The ESCRT-III-like protein Vipp1 couples filament polymerization with membrane remodeling. It assembles planar sheets as well as 3D rings and helical polymers, all implicated in mitigating plastid-associated membrane stress. PspA activity is triggered by agents that threaten inner membrane integrity, including phage, mislocalized secretins, and antibiotics, whereas Vipp1 is a plastid component in cyanobacteria, algae, and plants, in which it functions in thylakoid membrane biogenesis and repair. Given that two-dimensional (2D) planar sheets share a close geometric relationship with helical lattices, and as a means of understanding the interconnectedness of Vipp1 polymers including rings, spirals and planar sheets, we determined the structure of four Vipp1 helical filaments by cryo-EM.

Alternatively, Vipp1Δα61–219 assembled with related but different lattices, termed Vipp1Δα6_L2 and Vipp1Δα6_L3. Vipp1Δα6_L3 was the only lattice in which class averages of aligned particles yielded a Fourier Transform with non-overlapping layer lines amenable to indexing. Only helical parameters with a rise of 2.16 Å and a rotation of 85.50° yielded a 3.7 Å-resolution map, with excellent side chain detail enabling model building from amino acids 1–217. Map quality was lowest around the C terminus of helix 5 (α5C), indicative of instability within interface 1—a trait observed for all Vipp1 helical filaments, to differing degrees. Vipp1Δα6_L3 was 24.4 nm in diameter, with a hollow inner lumen that was 12.7 nm across. Specifically, Vipp1 formed ESCRT-III-like protofilaments, in which hairpin motifs packed side by side and the α5C of subunit j bound across the hairpin tip of subunit j+3 to form the classical interface 1 domain swop. These protofilaments formed a 17-start right-handed helix that ran diagonally around the helical axis. Concurrently, each hairpin tip bound the N terminus of helix 5 (α5N) in a neighboring protofilament, thereby forming interface 3. Neighboring protofilaments aligned laterally to form a 4-start left-handed helix, in which subunits connected through the stacking of helices α0 and the formation of interface 2. The 4-start helix has a pitch of 44 Å and forms diagonal parallel ridges that encircle the helical axis and dominate the surface topology of the Vipp1 helical filament.

> MGLFDRIKRVVSSNLNDLVNKAEDPEKMLEQAILEMQEDLVQLRQGVAQAIAAQKRSEKQYNDAQNEINKWQRNAQLALQKGDENLARQALERKKTYTDTSAALKASLDTQSTQVETLKRNLIQLESKISEAKTKKEMLKARITTAKAQEQLQGMVRGMNTSSAMSAFERMEEKVLMQESRAQALGELAGADLETQFAQLEGGSDVDDELAALKAQMLP> MVGADLGLWNRLEPALAYLAPEERAKVREAYRFAEEAHRGQLRRSGEPYITHPVAVAEILAGLQMDADTVAAGLLHDTLEDCGVAPEELERRFGPTVRRIVEGETKVSKLYKLANLEGEERRAEDLRQMFIAMAEDVRIIIVKLADR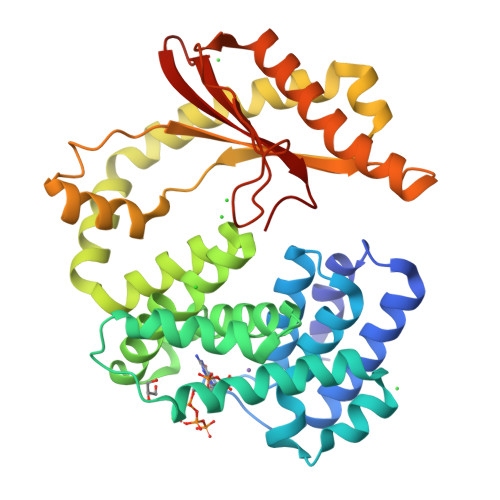LHNLRTLEHMPPEKQKRIAQETLEIYAPLAHRLGMGQLKWELEDLSFRYLHPEAFASLSARIQATQEARERLIQKAIHLLQETLARDELLQSQLQGFEVTGRPKHLYSIWKKMEREGKTLEQIYDLLAVRVILDPKPAPTRESQALREKQVCYHVLGLVHALWQPIPGRVKDYIAVPKPNGYQSLHTTVIALEGLPLEVQIRTREMHR>AGCSSYVIINTRGTSEPQGPSVGFRTMNTRIRSAVSGGSEYDTVYPAGIDQNSAQGTANIVAQVKAGLARNPNTCFLLEGYSQGAAATCNALPQLTGAAFDAVKGVILIGNPEHKPNLACNVDGNGGKTTFSARGISAAFTQGVPSNWVSKTLDICIYGDGVCDVSSGFGITPQHLTYGY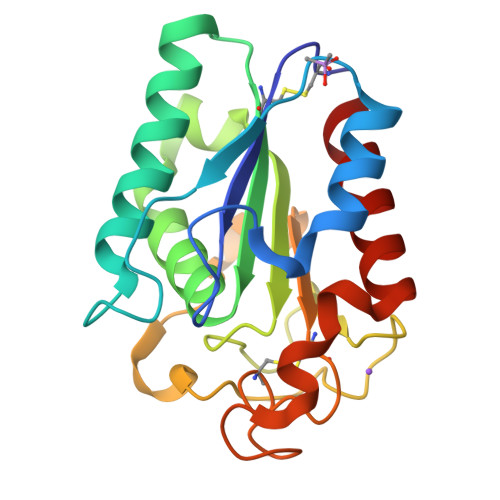NTNVQTMGANFGIKALQG[2x]CRISPR–Cas adaptive immune systems capture DNA fragments from invading mobile genetic elements and integrate them into the host genome to provide a template for RNA-guided immunity. Here we reconstitute CRISPR sequence capture, processing and integration by a naturally occurring Megasphaera NM10-related Cas2 and DEDDh fusion protein (Cas2/DEDDh) in complex with Cas1 (Cas1–Cas2/DEDDh). The natural Cas1–Cas2/exonuclease fusion (trimmer-integrase) catalyses coordinated DNA capture, trimming and integration. The Megasphaera Cas1–Cas2 retains the canonical heterohexameric architecture, with two Cas1 dimers (denoted Cas1 and Cas1′, a or b subunit) bridged by a central Cas2 dimer.

Aiming to visualize DEDDh trimming and conformational changes in Cas1, we used cryo-EM to characterize Cas1–Cas2/DEDDh in complex with a DNA half-site analogue containing phosphorothioate linkages at the PAM positions. Neither the initial 3.1 Å density nor any heterogeneous states detected during cryo-EM data processing had density corresponding to the DEDDh domain on the PAM side of the complex. The 3.1 Å half-site structure reveals interactions at the first integration strand junction. The spacer-ligated first CRISPR repeat guanine G29 was found in two approximately equivalent conformations. In the first conformation, G29 forms a canonical base pair with C35 (Fig. 3d (middle)). In the second conformation, G29 flips upwards, making a specific contact with loop 7 lysine Lys168. The lysine also contacts the 3′ hydroxyl of the leader (Fig. 3d (left)). Gln141, which sits at the base of helix 7, also makes a nucleobase-specific contact with C35, the first bottom repeat nucleotide. The 3.1 Å half-site complex reconstruction contains density corresponding only to the leader-proximal region of the CRISPR repeat.

>MPMTVITLKNVPQSLRGDLTRWMQEIATGVYVGNFNSRIREYLWRRVQETMGAGEASMCFAARNELGYDFLTENASRSVIDYDGLPLIFIPKEQSAVSDLPKGFSTAAKLHRAHIAGSGKKKEKPIRYVVIDIETDGKDAKRNHILEIGAIRCEDGKETHFTALISGDAVPPSITKLTGITATLLQKEGQEEKKVLTAFREFIGDDDLVGYHVSFDIEFLRQAFKKYGLGYLKNKTHDLLRIVKKEQLFQADYKLETSLQSYGIHKKVPHRALGDAELVKCLAKKLNKF[2x];>[4x]MAGPIIAGKSESSELPRVEDRATFIYIEHAKINRVDSAVTVAEAKGVVRIPAAMIGVLLLGPGTDISHRAVELLGDTGTALVWVGEQGVRYYASGRALARSTRFLVKQAELVTNERSRLRVARRMYQMRFPTEDVSKLTMQQLRSHEGARVRRKYRELSKKYNVPWKKRVYNPDDFAGGDPINQALSAAHVALYGLVHSVVAALGLSPGLGFVHTGHDRSFIYDVADLYKAEITVPIAFAVAAEAEEGQDIGQLARLRTRDAFVDGKILKRMVKDLQTLLEIPEEGQIEAEPLSLWDDKEKLVPYGVNYSEVTSCP>MDFAVMKQVKNTGLLQSEELCQYILRTSVYPREAGFLKELREANESHPDSYMSTSPLAGQLMSFVLKLVNAKKTIEVGVFTGYSLLLTALSIPDDGKITAIDFDREAYEIGLPFIRKAGVEHKINFIESD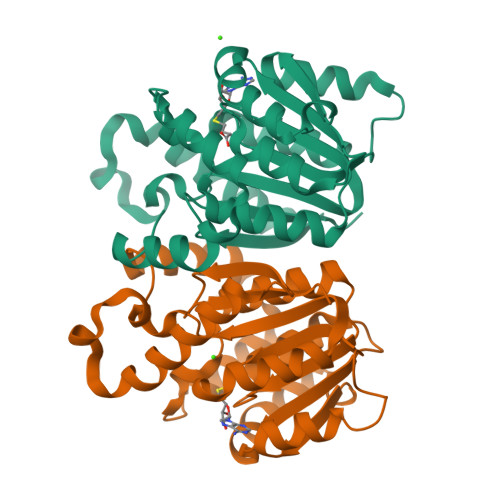AMLALDNLLQGQESEGSYDFGFVDADKPNYIKYHERLMKLVKVGGIVAYDNTLWGGTVAQPESEVPDFMKENREAVIELNKLLAADPRIEIVHLPLGDGITFCRRLY[2x]>ETLVRPKPELLKLLKSVGAQKDTYTMKEVLFYLGQYIMTKRLYDEKQQHIVYCSND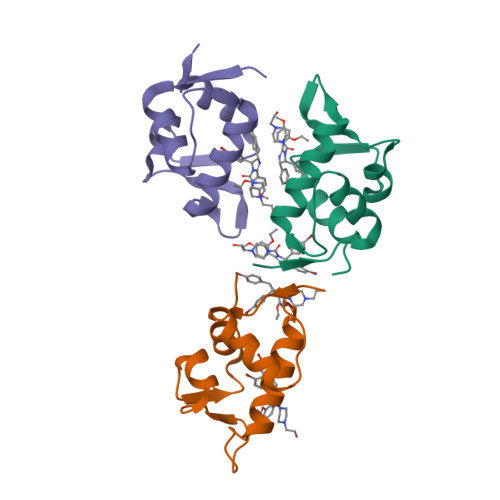LLGDLFGVPSFSVKEHRKIYTMIYRNLVV[3x]>[2x]SNAERTVADIMVPRSRMDLLDISQPLPQLLATIIETAHSRFPVYEDDRDNIIGILLAKDLLRYMLEPALDIRSLVRPAVFIPEVKRLNVLLREF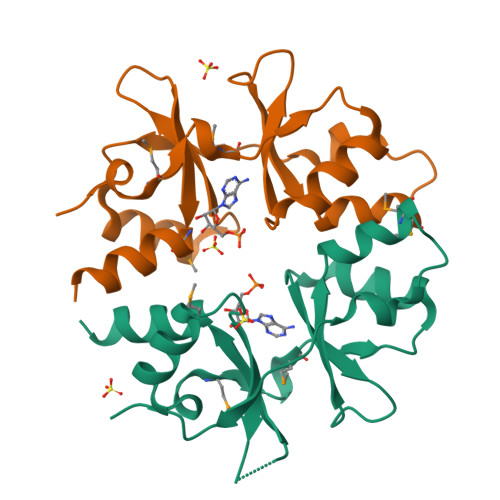RASRNHLAIVIDEHGGISGLVTMEDVLEQIVGDIE> SNAAIASEFSSLPSYAAFATAQEAYEQAVANGDSEVVLKKLKKSLNVAKSEFDRDAAMQRKLEKMADQAMTQMYKQARSEDKRAKVTSAMQTMLFTMLRKLDNDALNNIINNARDGCVPLNI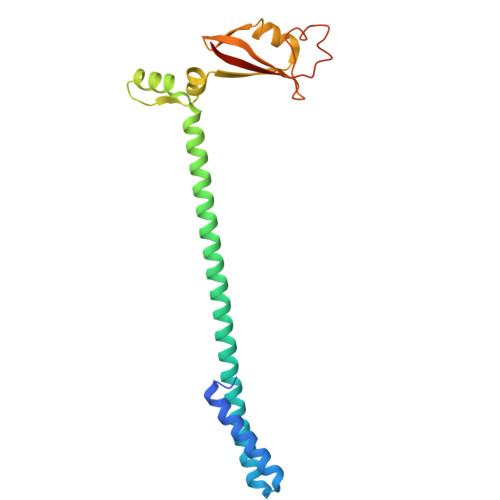IPLTTAAKLMVVIPDYNTYKNTCDGTTFTYASALWEIQQVVDADSKIVQLSEISMDNSPNLAWPLIVTALRANSAVKLQ1-(4-azanyl-3-methoxy-phenyl)ethanone | C9 H11 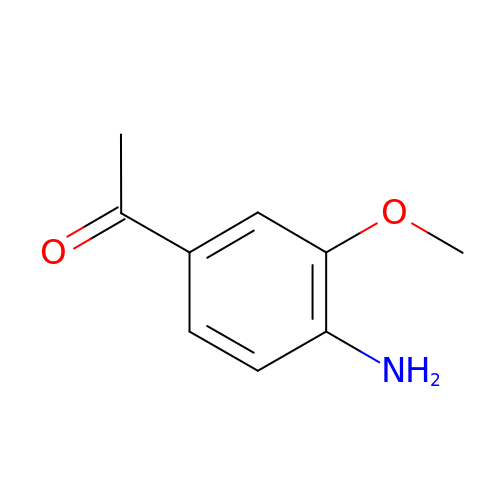N O2 | LNRPHCWGORQWPI-UHFFFAOYSA-N>[4x]PTIFEERHLKYISQLGKGNFGSVELCRYDPLGDNTGALVAVKQLQHSGPDQQRDFQREIQILKALHSDFIVKYRGVSYGPGRQSLRLVMEYLPSGCLRDFLQRHRARLDASRLLLYSSQICKGMEYLGSRRCVHRDLAARNILVESEAHVKIADFGLAKLLPLDKDYYVVREPGQSPIFWYAPESLSDNIFSRQSDVWSFGVVLYELFTYCDKSCSPSAEFLR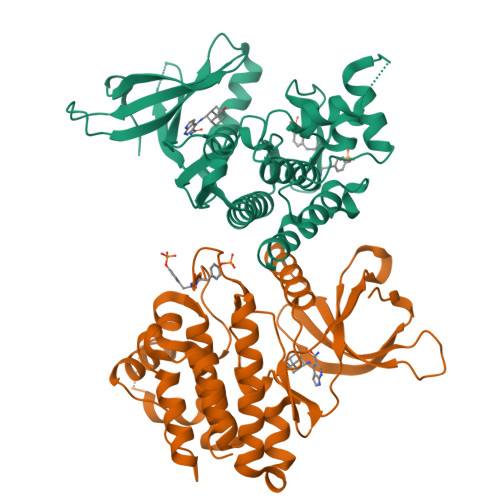MMGSERDVPALSRLLELLEEGQRLPAPPACPAEVHELMKLCWAPSPQDRPSFSALGPQLDMLWS>[3x]DRHHHHHHKLSPPAAPRFNVSLDSVPELRWLPVLRHYDLDLVRAAMAQVIGDRVPKWVHVLIGKVVLELERFLPQPFTGEIRGMCDFMNLSLADCLLVNLAYESSVF;>[3x]CTSIVAQDSRGHIYHGRNLDYPFGNVLRKLTVDVQFLKNGQIAFTGTTFIGYVGLWTGQSPHKFTVSGDERDKGWWWENAIAAL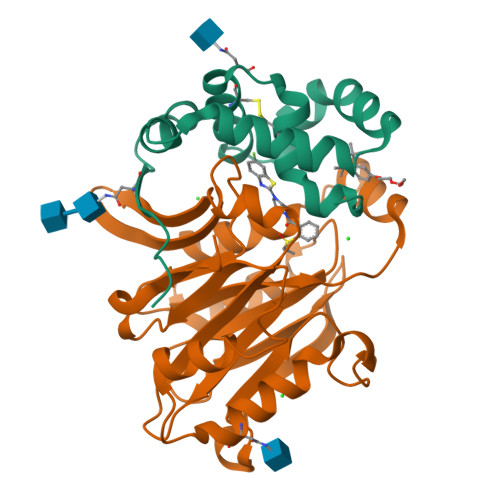FRRHIPVSWLIRATLSESENFEAAVGKLAKTPLIADVYYIVGGTSPREGVVITRNRDGPADIWPLDPLNGAWFRVETNYDHWKPAPKEDDRRTSAIKALNATGQANLSLEALFQILSVVPVYNNFTIYTTVMSAGSPDKYMTRIRNPSRK> NAMAYSKIRQPKLSDVIEQQLEFLILEGTLRPGEKLPPERELAKQFDVSRPSL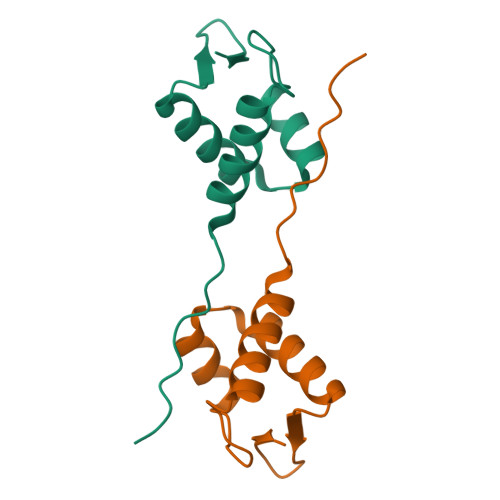REAIQRLEAKGLLLRRQGGGTFVQ>[2x]MGSSHHHHHHSS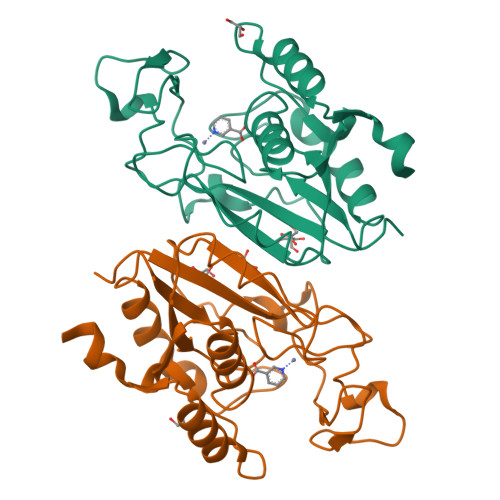GENLYFQGHMKMNKQPQNSALVVVDVQNGFTPGGNLAVADADTIIPTINQLAGCFENVVLTQDWHPDNHISFAANHPGKQPFETIELDYGSQVLWPKHCIQGTHDAEFHPDLNIPTAQLIIRKGFHAHIDSYSAFMEADHTTMTGLTGYLKERGIDTVYVVGIATDFCVAWTALDAVKQGFKTLVIEDACKGIDLNGSLEQAWQTMQQQGVVRIQSTDLLNEC>[3x]GMSPRVGVTLSGRYRLQRLIATGGMGQVWEAVDNRLGRRVAVKVLKSEFSSDPEFIERFRAEARTTAMLNHPGIASVHDYGES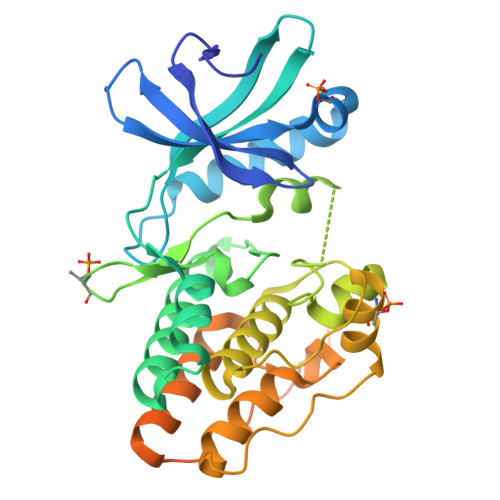QMNGEGRTAYLVMELVNGEPLNSVLKRTGRLSLRHALDMLEQTGRALQIAHAAGLVHRDVKPGNILITPTGQVKITDFGIAKAVDAAPVTQTGMVMGTAQYIAPEQALGHDASPASDVYSLGVVGYEAVSGKRPFAGDGALTVAMKHIKEPPPPLPPDLPPNVRELIEITLVKNPAMRYRSGGPFADAVAAVRAGRRPPRPSQTPPPGRAAPAAIPSGTTARVAANSAGRTAASRRSRPATGGHRPPRRTFSSG> GHMLQNNTDYPFEANNPYMYHENPMEEGLSMLKLANLAEAALAFEAVCQAAPEREEAWRSLGLTQAENEKDGLAIIALNHARMLDPKDIAVHAALAVSHTNEHNANAALASLRAWLLSQPQYEQLGSVNLQADVDIDDLNVQSEDFFFAAPNEYRECRTLLHAALEMNPNDAQLHASLGVLYNLSNNYDSAAANLRRAVELRPDDAQLWNKLGATLANGNRPQEALDAYNRALDINPGYVRVMYNMAV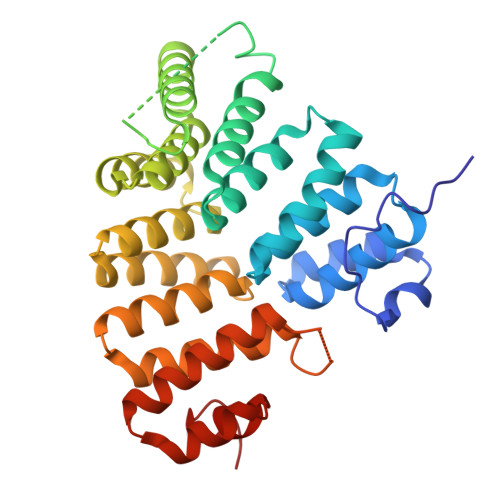SYSNMSQYDLAAKQLVRAIYMQVGGTTPTGEASREATRSMWDFFRMLLNVMNRPDLVELTYAQNVEPFAKEFGLQSMLL>[2x]HHHHHHFNLPPGNYKKPKLLYCSNGGHFLRIAPDGTVDGTRDRSDQHIQLQLSAESVGEVYIKSTETGQYLAMDTDG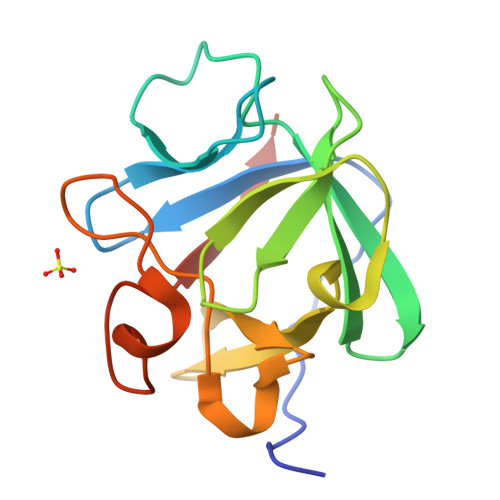LLYGSQTPNEECLFLERLEENHYNTYISKKHAEKNWFVGLKKNGSCKRGPRTHYGQKAILFLPLPVSSD> GLPVCGETCVG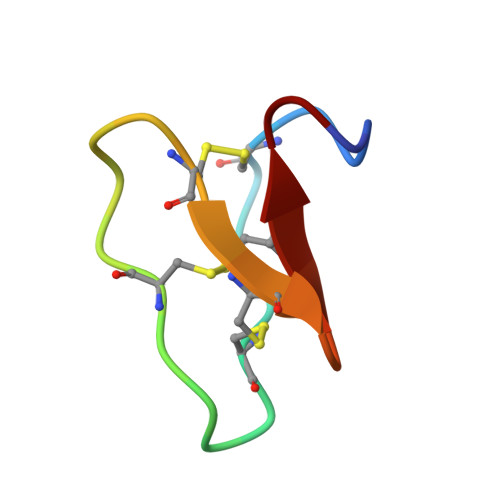GTCNTPGCTCSWPVCTRN>SRTIGIIGAPFSKGQPRGGVEEGPTVLRKAGLLEKLKEQECDVKDYGDLPFADIPNDSPFQIVKNPRSVGKASEQLAGKVAEVKKNGRISLVLGGDHSLAIGSISGHARVHPDLGVIWVDAHT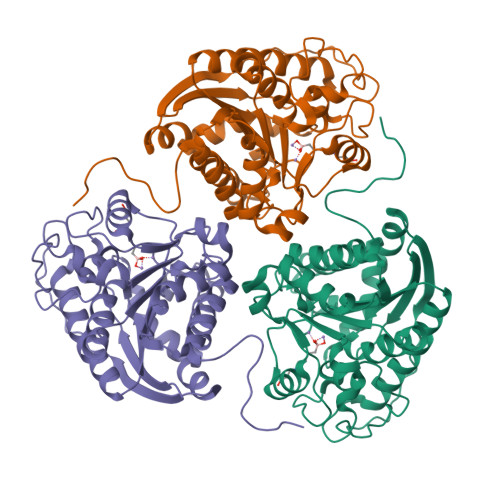DINTPLTTTSGNLHGQPVSFLLKELKGKIPDVPGFSWVTPCISAKDIVYIGLRDVDPGEHYILKTLGIKYFSMTEVDRLGIGKVMEETLSYLLGRKKRPIHLSFDVDGLDPSFTPATGTPVVGGLTYREGLYITEEIYKTGLLSGLDIMEVNPSLGKTPEEVTRTVNTAVAITLACFGLAREGNHKPIDYL[2x]> 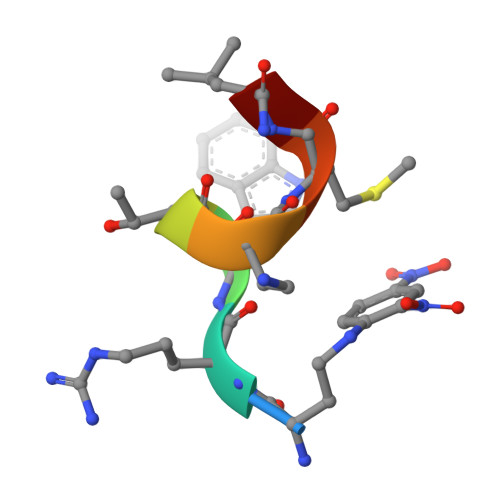XRWTAMLG> MQLKRVAEAKLPTPWGDFLMVGFEELATGHDHVALVYGDISGHTPVLARVHSECLTGDALFSLRCDCGFQLE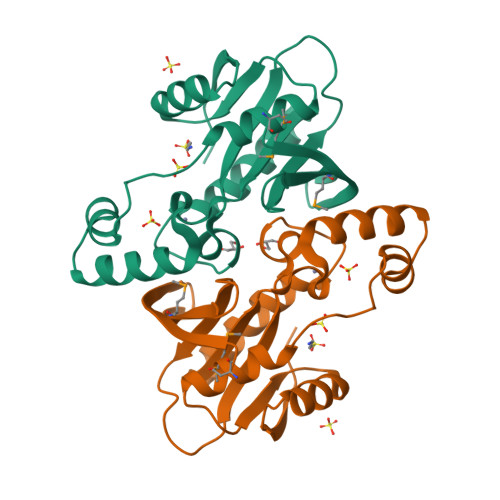AALTQIAEEGRGILLYHRQEGRNIGLLNKIRAYALQDQGYDTVEANHQLGFAADERDFTLCADMFKLLGVNEVRLLTNNPKKVEILTEAGINIVERVPLIVGRNPNNEHYLDTKAEKMGHLLNK pmcCyclophilins (Cyps) are ubiquitous and evolutionarily well-conserved proteins first recognized as specific cellular receptors for the immunosuppressant cyclosporin A (CsA). These proteins are endowed with peptidyl-prolyl isomerase (PPIAse) activity to catalyze trans-to-cis isomerization of peptide bonds at proline residues, which is a critical step for correct protein folding. Herein, we characterize the functional and structural properties of a conserved (TgCyp23) and a more divergent (TgCyp18.4) cyclophilin isoform from T. gondii. While TgCyp23 is a highly active cis–trans-prolyl isomerase (PPIase) and binds CsA with nanomolar affinity, TgCyp18.4 shows low PPIase activity and is significantly less sensitive to CsA inhibition.

There are two monomers in the asymmetric unit with an almost identical structure (RMSD of 0.109 Å for the Cα superposition). The overall structure of TgCyp23 follows the folding observed in the Cyps family and is composed of a β-barrel of eight antiparallel β-strands with two α-helices on the bottom and top of the barrel, all connected by loops. As observed, the Cyp folding is preserved, with main differences in TgCyp23 related to the 40 extra residues in the N-terminal region. The residues constituting the binding pocket are Arg99, Phe104, Met105, Gln106, Ala145, Asn146, Ser147, Gln155, Phe157, Trp165, Leu166, and His170. Stabilization of CsA is performed mainly by polar interactions and van der Waals forces. Trp165 residue, located in a 310-helix in the Lβ6β7 loop, is crucial in CsA stabilization due to the formation of a hydrogen bond between its NE1 and the carbonyl O atom of MLE-2 in CsA. Gln107 plays a very important role in the CsA packaging since it both establishes a H-bond interaction with CsA and acts as a bridging residue in a H-bond network that stabilizes the proper orientation of nearby residues Arg99 and Gln155. Interestingly, this pattern is preserved in TgCyp23, and the same polypeptide substrate nicely accommodates into its active site by the direct superimposition of CypA onto TgCyp23. Both the hydrophobic pocket (Ile101, Phe104, Met105, Ala145, Phe157, Leu166) and the catalytic arginine (Arg99) are conserved as well as residues in the H-bond network, providing a substrate-binding site with similar shape and dimensions.

>MAPAPPANSGESSLLSESELPAGISYAEAMEGGSRPLLHPDNPVVFFDISIGSHEAGRIKIELFKNLAPKSAENFRQFCTGEFRQNQVPIGYKGATFHRIIKNFMIQGGDFVKGDGTGRLSIYGSSFPDEAFVLPHFRSGLLSLANSGPDTNGCQFFITCAKCDWLNRKHVVFGQVLGKESMQVVRKIEHVTVDGGNRPRIPVTVTQCGEL[2x];>[2x]ALLVTAGLVLA5-{[(3-phenoxyphenyl)methyl][(1S)-1,2,3,4-tetrahydronaphthalen-1-yl]carbamoyl}benzene-1,2,4-tricarboxylic acid | C33 H27 N O8 | 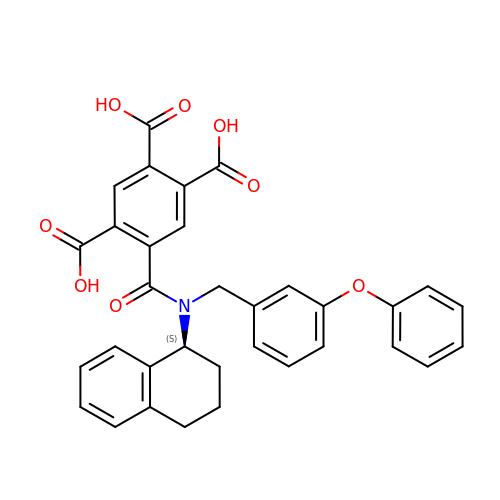VQGBOYBIENNKMI-LJAQVGFWSA-N> MDLNDLPMDVF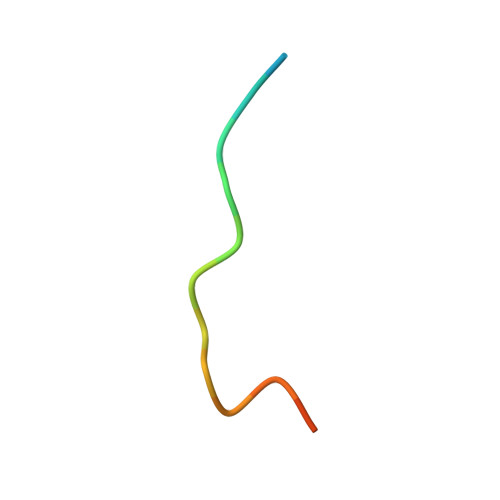ELADS> XXXXXXXXXXXXXXXXXXXXXXXXXXXXXXXXXXXXXXXXXXXXXXXXXXXXXXXXXXXXXXXXXXXXXXXXXXXXXXXXXXXXXXXXXXXXXXXXXXXXXXXXXXXXXXXXXXXXXXXXXXXXXXXXXXXXXXXXXXXXXXXXXXXXXXXXXXXXXXXXXXXXXXXXXXXXXXXXXXXXXXXXXXXXXXPSVPECFTIEKKSSYFIIEPQDLSTKVASICGVIVPKVHTIHDKVFYPLTFVPTHKTVSSLRQLGRKIQNSTPIMLIGKAGSGKTFLINELSKYMGCHDSIVKIHLGEQTDAKLLIGTYTSGDKPGTFEWRAGVLATAVKEGRWVLIEDIDKAPTDVLSILLSLLEKRELTIPSRGETVKAANGFQLISTVRINEDHQKDSSNKIYNLNMIGMRIWNVIELEEPSEEDLTHILAQKFPILTNLIPKLIDSYKNVKSIYMNTKFISLNKGAHTRVVSVRDLIKLCERLDILFKNNGINKPDQLIQSSVYDSIFSEAADCFAGAIGEFKALEPIIQAIGESLDIASSRISLFLTQHVPTLENLDDSIKIGRAVLLKEKLNIQKKSMNSTLFAFTNHSLRLMEQISVCIQMTEPVLLVGETGTGKTTVVQQLAKMLAKKLTVINVSQQTETGDLLGGYKPVNSKTVAVPIQENFETLFNATFSLKKNEKFHKMLHRCFNKNQWKNVVKLWNEAYKMAQSILKITNTENENENAKKKKRRLNTHEKKLLLDKWADFNDSVKKFEAQSSSIENSFVFNFVEGSLVKTIRAGEWLLLDEVNLATADTLESISDLLTEPDSRSILLSEKGDAEPIKAHPDFRIFACMNPATDVGKRDLPMGIRSRFTEIYVHSPERDITDLLSIIDKYIGKYSVSDEWVGNDIAELYLEAKKLSDNNTIVDGSNQKPHFSIRTLTRTLLYVTDIIHIYGLRRSLYDGFCMSFLTLLDQKSEAILKPVIEKFTLGRLKNVKSIMSQTPPSPGPDYVQFKHYWMKKGPNTIQEQAHYIITPFVEKNMMNLVRATSGKRFPVLIQGPTSSGKTSMIKYLADITGHKFVRINNHEHTDLQEYLGTYVTDDTGKLSFKEGVLVEALRKGYWIVLDELNLAPTDVLEALNRLLDDNRELFIPETQEVVHPHPDFLLFATQNPPGIYGGRKILSRAFRNRFLELHFDDIPQDELEIILRERCQIAPSYAKKIVEVYRQLSIERSASRLFEQKNSFATLRDLFRWALRDAVGYEQLAA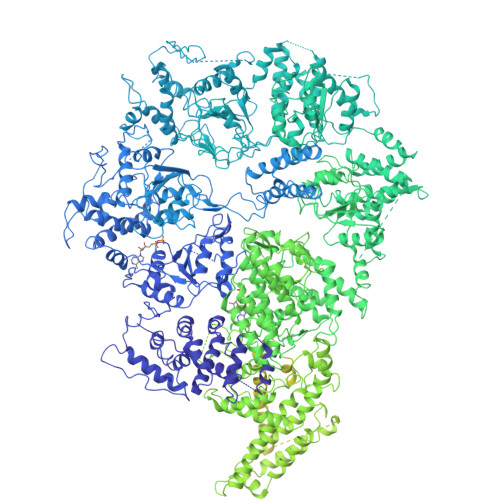SGYMLLAERCRTPQEKVTVKKTLEKVMKVKLDMDQYYASLEDKSLEAIGSVTWTKGMRRLSVLVSSCLKNKEPVLLVGETGCGKTTICQLLAQFMGRELITLNAHQNTETGDILGAQRPVRNRSEIQYKLIKSLKTALNIANDQDVDLKELLQLYSKSDNKNIAEDVQLEIQKLRDSLNVLFEWSDGPLIQAMRTGNFFLLDEISLADDSVLERLNSVLEPERSLLLAEQGSSDSLVTASENFQFFATMNPGGDYGKKELSPALRNRFTEIWVPSMEDFNDVNMIVSSRLLEDLKDLANPIVKFSEWFGKKLGGGNATSGVISLRDILAWVEFINKVFPKIQNKSTALIQGASMVFIDALGTNNTAYLAENENDLKSLRTECIIQLLKLCGDDLELQQIETNEIIVTQDELQVGMFKIPRFPDAQSSSFNLTAPTTASNLVRVVRAMQVHKPILLEGSPGVGKTSLITALANITGNKLTRINLSEQTDLVDLFGADAPGERSGEFLWHDAPFLRAMKKGEWVLLDEMNLASQSVLEGLNACLDHRGEAYIPELDISFSCHPNFLVFAAQNPQYQGGGRKGLPKSFVNRFSVVFIDMLTSDDLLLIAKHLYPSIEPDIIAKMIKLMSTLEDQVCKRKLWGNSGSPWEFNLRDTLRWLKLLNQYSICEDVDVFDFVDIIVKQRFRTISDKNKAQLLIEDIFGKFSTKENFFKLTEDYVQINNEVALRNPHYRYPITQNLFPLECNVAVYESVLKAINNNWPLVLVGPSNSGKTETIRFLASILGPRVDVFSMNSDIDSMDILGGYEQVDLTRQISYITEELTNIVREIISMNMKLSPNATAIMEGLNLLKYLLNNIVTPEKFQDFRNRFNRFFSHLEGHPLLKTMSMNIEKMTEIITKEASVKFEWFDGMLVKAVEKGHWLILDNANLCSPSVLDRLNSLLEIDGSLLINECSQEDGQPRVLKPHPNFRLFLTMDPKYGELSRAMRNRGVEIYIDELHSRSTAFDRLTLGFELGENIDFVSIDDGIKKIKLNEPDMSIPLKHYVPSYLSRPCIFAQVHDILLLSDEEPIEESLAAVIPISHLGEVGKWANNVLNCTEYSEKKIAERLYVFITFLTDMGVLEKINNLYKPANLKFQKALGLHDKQLTEETVSLTLNEYVLPTVSKYSDKIKSPESLYLLSSLRLLLNSLNALKLINEKSTHGKIDELTYIELSAAAFNGRHLKNIPRIPIFCILYNILTVMSENLKTESLFCGSNQYQYYWDLLVIVIAALETAVTKDEARLRVYKELIDSWIASVKSKSDIEITPFLNINLEFTDVLQLSRGHSITLLWDIFRKNYPTTSNSWLAFEKLINLSEKFDKVRLLQFSESYNSIKDLMDVFRLLNDDVLNNKLSEFNLLLSKLEDGINELELISNKFLNKRKHYFADEFDNLIRYTFSVDTAELIKELAPASSLATQKLTKLITNKYNYPPIFDVLWTEKNAKLTSFTSTIFSSQFLEDVVRKSNNLKSFSGNQIKQSISDAELLLSSTIKCSPNLLKSQMEYYKNMLLSWLRKVIDIHVGGDCLKLTLKELCSLIEEKTASETRVTFAEYIFPALDLAESSKSLEELGEAWITFGTGLLLLFVPDSPYDPAIHDYVLYDLFLKTKTFSQNLMKSWRNVRKVISGDEEIFTEKLINTISDDDAPQSPRVYRTGMSIDSLFDEWMAFLSSTMSSRQIKELVSSYKCNSDQSDRRLEMLQQNSAHFLNRLESGYSKFADLNDILAGYIYSINFGFDLLKLQKSKDRASFQISPLWSMDPINISCAENVLSAYHELSRFFKKGDMEDTSIEKVLMYFLTLFKFHKRDTNLLEIFEAALYTLYSRWSVRRFRQEQEENEKSNMFKFNDNSDDYEADFRKLFPDYEDTALVTNEKDISSPENLDDIYFKLADTYISVFDKDHDANFSSELKSGAIITTILSEDLKNTRIEELKSGSLSAVINTLDAETQSFKNTEVFGNIDFYHDFSIPEFQKAGDIIETVLKSVLKLLKQWPEHATLKELYRVSQEFLNYPIKTPLARQLQKIEQIYTYLAEWEKYASSEVSLNNTVKLITDLIVSWRKLELRTWKGLFNSEDAKTRKSIGKWWFYLYESIVISNFVSEKKETAPNATLLVSSLNLFFSKSTLGEFNARLDLVKAFYKHIQLIGLRSSKIAGLLHNTIKFYYQFKPLIDERITNGKKSLEKEIDDIILLASWKDVNVDALKQSSRKSHNNLYKIVRKYRDLLNGDAKTIIEAGLLYSNENKLKLPTLKQHFYEDPNLEASKNLVKEISTWSMRAAPLRNIDTVASNMDSYLEKISSQEFPNFADLASDFYAEAERLRKETPNVYTKENKKRLAYLKTQKSKLLGDALKELRRIGLKVNFREDIQKVQSSTTTILANIAPFNNEYLNSSDAFFFKILDLLPKLRSAASNPSDDIPVAAIERGMALAQSLMFSLITVRHPLSEFTNDYCKINGMMLDLEHFTCLKGDIVHSSLKANVDNVRLFEKWLPSLLDYAAQTLSVISKYSATSEQQKILLDAKSTLSSFFVHFNSSRIFDSSFIESYSRFELFINELLKKLENAKETGNAFVFDIIIEWIKANKGGPIKKEQKRGPSVEDVEQAFRRTFTSIILSFQKVIGDGIESISETDDNWLSASFKKVMVNVKLLRSSVVSKNIETALSLLKDFDFTTTESIYVKSVISFTLPVITRYYNAMTVVLERSRIYYTNTSRGMYILSTILHSLAKNGFCSPQPPSEEVDDKNLQEGTGLGDGEGAQNNNKDVEQDEDLTEDAQNENKEQQDKDERDDENEDDAVEMEGDMAGELEDLSNGEENDDEDTDSEEEELDEEIDDLNEDDPNAIDDKMWDDKASDNSKEKDTDQNLDGKNQEEDVQAAENDEQQRDNKEGGDEDPNAPEDGDEEIENDENAEEENDVGEQEDEVKDEEGEDLEANVPEIETLDLPEDMNLDSEHEESDEDVDMSDGMPDDLNKEEVGNEDEEVKQESGIESDNENDEPGPEEDAGETETALDEEEGAEEDVDMTNDEGKEDEENGPEEQAMSDEEELKQDAAMEENKEKGGEQNTEGLDGVEEKADTEDIDQEAAVQQDSGSKGAGADATDTQEQDDVGGSGTTQNTYEEDQEDVTKNNEESREEATAALKQLGDSMKEYHRRRQDIKEAQTNGEEDENLEKNNERPDEFEHVEGANTETDTQALGSATQDQLQTIDEDMAIDDDREEQEVDQKELVEDADDEKMDIDEEEMLSDIDAHDANNDVDSKKSGFIGKRKSEEDFENELSNEHFSADQEDDSEIQSLIENIEDNPPDASASLTPERSLEESRELWHKSEISTADLVSRLGEQLRLILEPTLATKLKGDYKTGKRLNMKRIIPYIASQFRKDKIWLRRTKPSKRQYQIMIALDDSKSMSESKCVKLAFDSLCLVSKTLTQLEAGGLSIVKFGENIKEVHSFDQQFSNESGARAFQWFGFQETKTDVKKLVAESTKIFERARAMVHNDQWQLEIVISDGICEDHETIQKLVRRARENKIMLVFVIIDGITSNESILDMSQVNYIPDQYGNPQLKITKYLDTFPFEFYVVVHDISELPEMLSLILRQYFTDLASS> LGSSNDNIELVDFQNIMFYGDAEVGDNQQPFTFILDTGSANLWVPSVKCTTAGCLTKHLYDSSKSRTYEKDGTKVEMNYVSGTVSGFFSKDLVTVGNLSLPYKFIEVIDTNGFEPTYTASTFDGILGLGWKDLSIGSVDPIVVELKNQNKIENALFTFYLPVHDKHTGFLTIGGIEERFYEGPLTYEKLNHDLYWQITLDA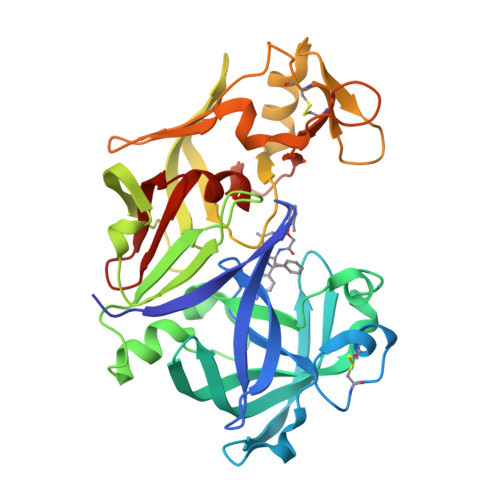HVGNISLEKANCIVDSGTSAITVPTDFLNKMLQNLDVIKVPFLPFYVTLCNNSKLPTFEFTSENGKYTLEPEYYLQHIEDVGPGLCMLNIIGLDFPVPTFILGDPFMRKYFTVFDYDNHSVGIALAKKNL> A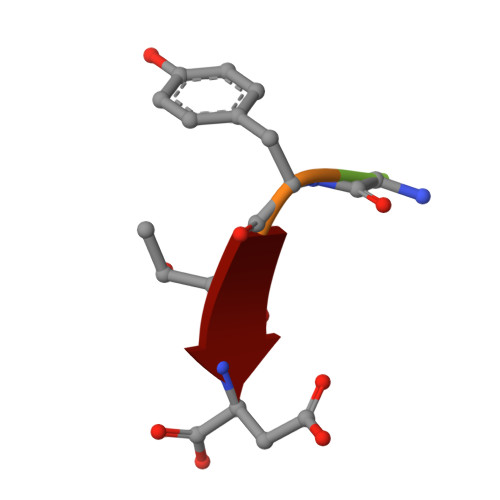GYTD> MNIHEYQAKAIFVDNGIPTLKGKVAFSVDEAVANAKELGGSVWAVKAQIHAGGRGLGGGVKIAKNLDEVKDYASKILGMNLVTHQTGPEGKLVQKLYIESGANIVKEYYLAILFNRMAEQITIIASSEGGMDIEKVAKESPEKIAKVGIDPQIGFKMFHGLEVARVLGLDKDEGKKLISMIAKLYKLYMDKDMNMLEINPLIKTAEGDFYALDAKCSFDDSALYRHPEIAELRDTTEENPAEREAAEFGLSYVKLDGDVACMVNGAGLAMATMDIINYSGAKPANFLDVGGGASPETVAKAFEIILRDKNVKVIFINIFGGIVRCDRIANGILEATKNVEVNIPIVVRLDGTNAAEAKTILDNSNLKNIKA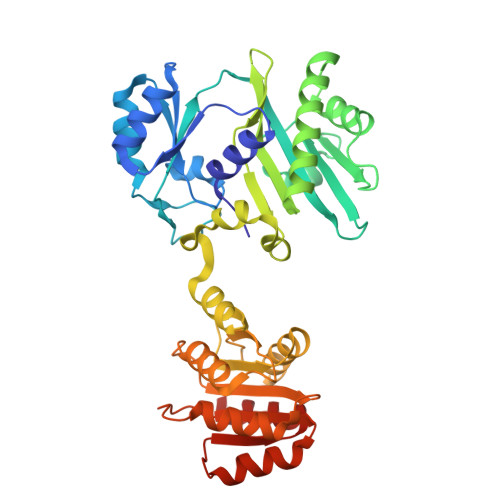ATNLKNGAELVKSLVG> AKPTKVTLVKSAKNEE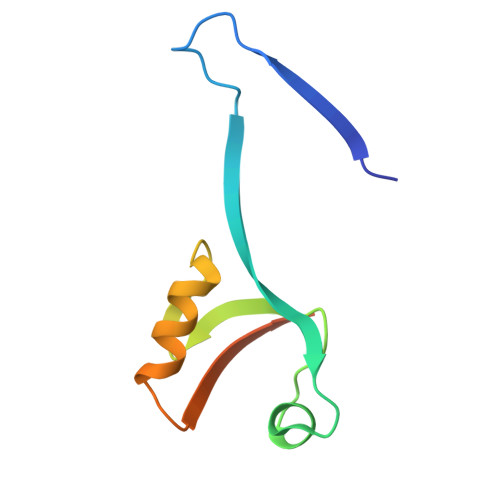YGLRLASHIFVKEISQDSLAARDGNIQEGDVVLKINGTVTENMSLTDAKTLIERSKGKLKMVVQRDERATLLNVPD>[4x]MGHHHHHHMAQKPVDNITQIIGGTPVVKLRNVVD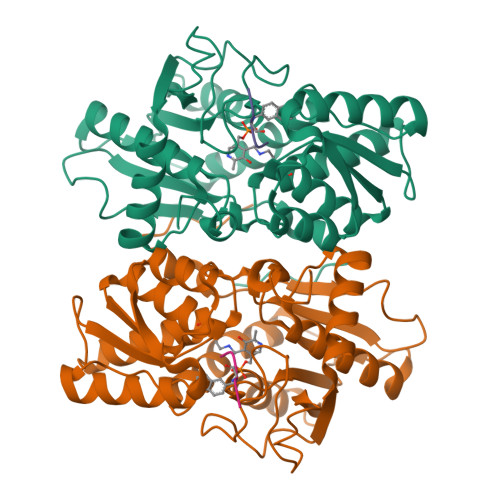DNAADVYVKLEYQNPGGSVKDRIALAMIEKAEREGKIKPGDTIVEPTSGNTGIGLAFVCAAKGYKAVFTMPETMSQERRNLLKAYGAELVLTPGSEAMKGAIKKAKELKEEHGYFEPQQFENPANPEVHELTTGPELLQQFEGKTIDAFLAGVGTGGTLSGVGKVLKKEYPNIEIVAIEPEASPVLSGGEPGPHKLQGLGAGFIPGTLNTEIYDSIIKVGNDTAMEMSRRVAKEEGILAGISSGAAIYAAIQKAKELGKGKTVVTVLPSNGERYLSTPLYSFDD;>[4x]YMAYI>[2x]KHSLPDL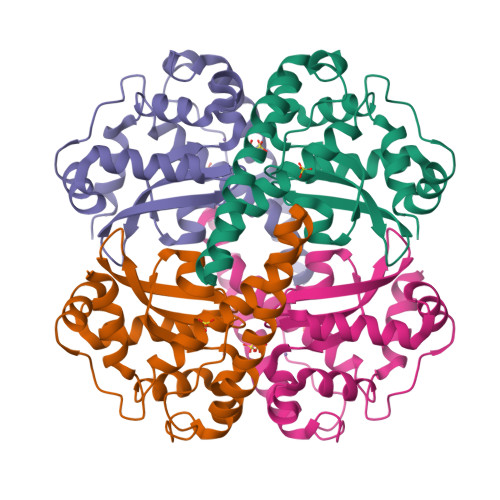PYDYGALEPHINAQIMQLHHSKHHAAYVNNLNVTEEKYQEALAKGDVTAQIALQPALKFNGGGHINHSIFWTNLSPNGGGEPKGELLEAIKRDFGSFDKFKEKLTAASVGVQGSGWGWLGFNKERGHLQIAACPNQDPLQGTTGLIPLLGIDVAEHAYYLQYKNVRPDYLKAIWNVINWENVTERYMACKK2-azanyl-8-[(4-chlorophenyl)methylsulfanyl]-1,9-dihydropurin-6-one | C12 H10 Cl N5 O S | 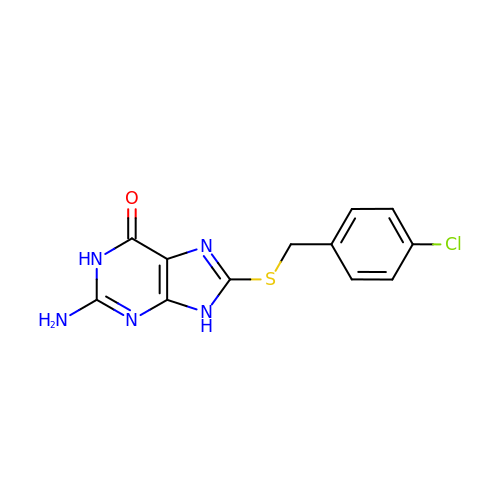MVZVAYOBERRXEC-UHFFFAOYSA-N BuV1 is a member of the Protoparvovirus genus of the Parvoviridae family. Similar to all known parvoviruses, BuV1 assembles into a T = 1 icosahedral capsid. The gross capsid morphology includes pores at the 5-fold vertices, protrusions surrounding the 3-fold axes, a depression region at the 2-fold axes, and a wall separating the depressed regions near the 2- and 5-fold axes. The VPs have an eight-stranded β-barrel motif and an α-helix that form the core of the capsid, which is characteristic of all members of the Parvoviridae.

In order to characterize the structural rearrangements that may occur under various pHs relevant to the viral lifecycle, BuV1 capsids were dialyzed to pH 7.4, 4.0, or 2.6, vitrified on cryo-EM grids, and subjected to cryo-EM data collection. Subsequent 3D reconstruction yielded electron density maps at 2.84, 3.20, and 2.73 Å for pH 7.4, 4.0, and 2.6, respectively. At pH 2.6, the ordering of the N-terminus allowed for the assignment of 10 additional residues compared to either pH 7.4 or 4.0 structures. However, reasonable electron density allowed the fitting of this loop at pH 2.6. For instance, the large rearrangement in VR-IX observed at pH 2.6 occurs at the 2-fold axis of symmetry, which suggests that this may destabilize the 2-fold interface. Indeed, in micrographs of the BuV1 capsid at pH 2.6, capsids were observed that appeared “broken” (red arrow). The ordering of additional residues at the N-terminal was also observed at pH 2.6, similar to the HBoV1 and HBoV2 capsids. At pH 7.4 and 2.6, the rotamer is in an extended conformation, resulting in a pore with an approximate radius of 3.8 Å. At pH 2.6, when the virus is presumably in the stomach, Q157 adopts an extended conformation that restricts the radius of the 5-fold pore, preventing premature externalization of VP1u or the viral genome. The cryo-EM micrographs clearly show both full and half (broken) capsids at this pH; therefore, it is unclear whether the lack of signal is due to the fluorescent dye or if some of the hydrophobic patches of the capsid are exposed before heating.

>[60x]MPAIRKARGWVPPGYNYLGPFNQDFNKKPTNPSDNAARKHDLEYNKLIKQGHNPYWNYNHADEDFIKETDQATDWGGKFGNFVFRAKRALAPELAPPAKKKTKTKHTEPEYSHKHIKAGTKRGKPFYLFVNLARKKARMTDTQDVSEQQSDQPSVASTNAKAGGGGGGGGSGVGHSTGNYNNRTEFYYHGDEVTIVCHSSRHIHLNMSESEEYKIYDTDRGPRFPTDQTLQGRDTINDSYHAQVETPWFLINPNSWGTWMNPADFQQLTTTCREVTLEHLDQTLDNIVIKTVSKQGSGAEETTQYNNDLTALLQVALDKSNQLPWVADNMYLDSLGYIPWRPCKLKQYSYHVNFWNTIDIISGPQQNQWQQVKKEIRWDDLQFTPIETTTEIDLLRTGDSWTSGPYKFNTKPTQLSYHWQSTRHTGSVHPTDPPNAIGQQGQNIRDINGWQWGDRSDPMSAATRVSNFHIGYSWPEWRIHYGSGGPAINPGAPFSQAPWSTDPQVRLTQGASEKAIFDYNHGDDDPAHRDQWWQNNLPITGQTNWAPKNAHQANLSSNVPSRQEFWTQDYHNTFGPFTAVDDVGIQYPWGAIWTKTPDTTHKPMMSAHAPFICKDGPPGQLLVKLAPNYTENLQTDGLGNNRIVTYATFWWTGKLILKGKLRLPRQFNLYNLPGRPRGTEAKKFLPNEIGHFELPFMPGRCMPNYTM Several studies have shown that the -AATT- and -TTAA- sequences have distinct physical and interaction properties, especially in terms of their different requirements for recognition in the minor groove. Heterocyclic compounds with the appropriate shape can stack with the walls of the minor groove in -AATT- and related sequences, but the wider groove in -TTAA- and -TATA- sequences reduces the stacking energetics. Both the -TTAA- and -TATA- sequences are very important in the human genome. Because of the importance of these -TTAA- and -TATA- sequences, the design of small molecules that can strongly and selectively bind to them is an important research priority. In this work, we report on the design compounds that exhibit selective binding to -TTAA- or -TATA- containing DNA minor groove sequences compared with other AT ones.

The crystallization conditions for the native structure were similar to those for the complex. Several studies have illustrated that A-tract sequences, such as -AAAA- or -AATT-, have narrow minor grooves with strongly coordinated water molecules (i.e., a spin of hydration) in the groove, while wider minor grooves are observed in sequences such as -TTAA- and -TATA- with less tendency to form coherent patterns of structured water molecules. As a result, the minor grooves at the -TTAA- sequences are more readily expanded to accommodate a dimer complex; (ii) there is a critical interplay between the ligand structures and DNA sequences; for example, DB2009 with two thiophenes exhibits a relatively weak monomer binding (KA = 0.1 × 107 M–1) with -TTAA-. The dynamic flexibility of the -TTAA- site allows it to open for dimer formation.

> GCTGCGTTAACGCAGC> GSMTVEQNVLQQSAAQKHQQTFLNQLREITGINDTQILQQALKDSNGNLELAVAFLTAKNAKTPQQEETTYYQTALPGNDRYISVGSQADTNVIDLTGDDKDDLQRAIALSLAESNRAFRETGITDEEQAISRVLEASIAENKACLKRTPTEVWRDSRNPYDRKRQDKAPVGLKNVGNTCWFSAVIQSLFNLLEFRRLVLNYKPPSNAQDLPRNQKEHRNLPFMRELRYLFALLVGTKRKYVDPSRAVEILKDAFKSNDSQQQDVSEFTHKLLDWLEDAFQMKAEEETDEEKPKNPMVELFYGRFLAVGVLEGKKFENTEMFGQYPLQVNGFKDLHECLEAAMIEGEIESLHSENSGKSGQEHWFTELPPVLTFELSRFEFNQALGRPEKIHNKLEFPQVLYLDRYMHRNREITRIKREEIKRLKDYLTVLQQRLERYLSYGSGPKRFPLVDVLQYALEFASSKPVCTSPVDDIDASSPPSGSIPSQTLPSTTEQQGALSSELPSTSPSSVAAISSRSVIHKPFTQSRIPPDLPMHPAPRHITEEELSVLESCLHRWRTEIENDTRDLQESISRIHRTIELMYSDKSMIQVPYRLHAVLVHEGQANAGHYWAYIFDHRESRWMKYNDIAVTKSSWEELVRDSFGGYRNASAYCLMYINDKAQFLIQEEFNKETGQPLVGIETLPPDLRDFVEEDNQRFEKELEEWDAQLAQKALQE

USP25 shows activity in hydrolyzing K48- and K63-linked polyubiquitin chains and is a target for different post-translational modifications including phosphorylation, SUMOylation, and ubiquitination. Human USP25 is a modular protein composed by three domains: an NTD (Met1 to Tyr159), a central USP-like domain (Asp160 to Glu714), and a CTD (Lys715 to Arg1055). Strikingly, the USP25 structure displays a homotetramer quaternary assembly and the catalytic domain can be divided in three differentiated subdomains: a general palm-like catalytic domain (USP-like), a long coiled-coil (LCC), and an “inhibitory loop” (IL-loop or IL). In our USP25 structure, each IL-loop inserts into the catalytic domain from another molecule of the tetramer, thus preventing substrate binding and thereby impairing USP25 activity.

Interestingly, only the tetramer assembly of USP25 gave rise to single crystals. Initial diffraction of the USP25 crystals was poor, never beyond 6 Å resolution; however, after conducting a lysine methylation protocol, diffraction was notably improved, and thus finally collecting a 3.28 Å resolution dataset. The crystals belonged to the I422 space group, and contained one molecule per asymmetric unit. The USP25 structure was solved by SAD using mercurial derivatives, three of which were located bound to three cysteine residues (one corresponding to the active site cysteine). The structure of USP25 reveals the presence of a homotetramer quaternary assembly composed by the interaction of four different USP25 molecules from the crystal lattice. PISA server analysis also predicts that the tetramer structure of USP25 (A4), with a buried surface area of 23,730 Å2, is formed by the assembly of two homodimers (2 × A2). Each homodimer composing the USP25 tetramer is comprised by an extended contact interface that includes approximately half of the LCC coiled-coil domain, forming a four-helix bundle motif, which would act as a dimerization hub between two USP-like catalytic domains, resembling a “pair of cherries” with the knot at the end of their stems. The LCC-IL-loop insertion domain also participates in the tetramer interface, but in contrast to the dimer, the interaction occurs with the catalytic domain of the opposite dimer. Two contact areas can be distinguished in the tetramer interface: between the extended IL-loop which is deeply inserted into the S1 ubiquitin-binding surface of the catalytic domain (c in green and Supplementary Figure 4c); and between the LCC1 “kink” motif with residues from the loop connecting β9–β10 strands of the catalytic domain (Fig. 4a in blue and Supplementary Figure 4b).>MEFGFWSALYIFVLTAFLGYELITRVPVILHTPLMSGSNFIHGVVVVGAMVVLGHAETGLEKLIGFLGVILGAANAAGGYAVTVRMLEMFERKPGQGGGR[2x];>[2x]MDLIQAAYFVVAILFIVGLKRMAHPTTAKSGIVWAGWGMVLAVLATFFWPGMGNFALILLALLLGSVVAWWAAVRVAMTDMPQMVAIYNGMGGGAAATIAAVELLKGAFENTGLMALAILGGLIGSVAFTGSLIAFAKLQGIMKSRPILFPGQKAVNALVLALTVVIGLSLLWNDATASIVLFFLLALLFGVLMTLPIGGGDMPVAISFYNAFTGMAVGFEGFAVGNPALMVAGTLVGAAGTLLTVLMARAMNRSVWSVLVGGFGVEQEAGEVKGSLKPIDVEDAAVMLAYAGKVVFVPGYGMALSQAQHKLKELADLLEARGVEVKFAIHPVAGRMPGHMNVLLAEAGVDYDKLKDLEEINPEFPTVDVAVVIGANDVVNPAARRPGSPLYGMPILDVDKAKNVIVIKRGQGKGFAGVENELFYAENTRMLYGDAQKVLTELIQALKRL;>MHHHHHHHHMVTVAVPKERAPGERRVALVPEVVARLVKGGARVRVERGAGEGAYHPDEAYQEAGAEVVERGELLKGAHLLFTVQPPPEDLIQALEPGAIVVGFVQPHKNLELVRALQAKKATVIAMELIPRITRAQSMDALSSQATVAGYLAAIHAARLSPRFFPMLTTAAGTIRPAKVMVMGVGVAGLMAIATAKRLGAQVFAYDVRKAALEQALSLGAKPIELPISAE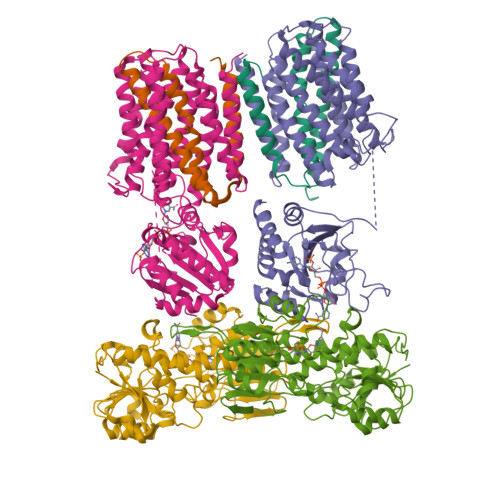GEGGYARELTEEEKRIQHEALRDHVAGMDVLITTAQVPGRRAPILLTEDMVERLKPGTVVVDLAAESGGNCVLTKPGEVVEVRGVRVYGPLNLPSELSVHASEMYAKNLYNLSSLLIEKGAFAPKWEDEIVRAALLMKEGEVLHGPTKALLGGA[2x]>SNAPGELKSVLRFKKLTEHAFTPSKGSKFAAGFDLCSAYDLVIPAVGKALVKTDIQVELPEG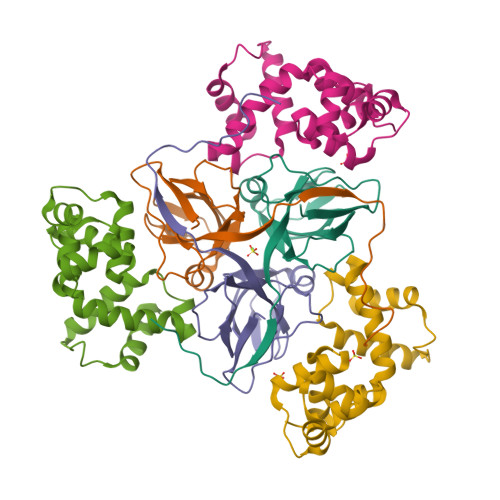CYGRIAPRSGLSWKHHIDVGAGVIDRDYRGNVGVVLFNHAKTDYEVKKGDRVAQLICEKIIYPEIQEVEELMETERGEGGFGSTGNQ[6x];>[6x]GAMEGAGQMAELPTHYGTIIKTLRKYMKLTQSKLSERTGFSQNTISNHENGNRNIGVNEIEIYGKGLGIPSYILHRISDEFKEKGYSPTLNDFGKFDKMYSYVNKAYYNDGDIYYSSYDLYDETIKLLELLKESKINVNDIDYDYVLKLYKQILSTD>MASGMIVTDAGADQPIVFVNRAFSTITGYAPNEVLGRNCRFLQGPQTDAATVARLREAIAAARPIQERILNYRK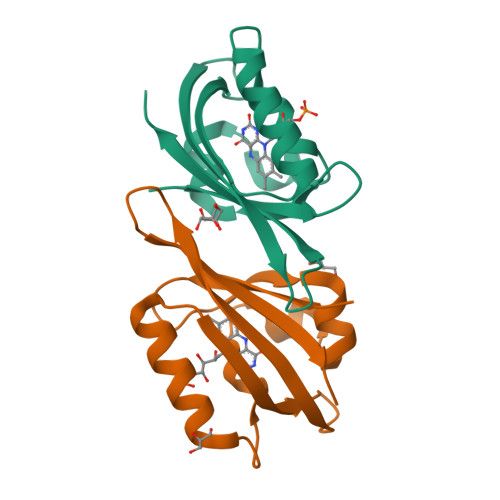DGQPFWNQLSISPVRDETGNVVAFVGVQTDVTAHHHHHH[2x]> AKMAFTLADRVTEEMLADKAALVVEVVEENYHDAPIVGIAVVNEHGRFFLRPETALADPQFVAWLGDETKKKSMFDSKRAAVALKWKGIELCGVSFDLLLAAYLLDPAQGVDDVAAAAKMKQYEAVRPDEAVYGKGAKRAVPDEPVLAEHLVRKAAAIWELERPFLDELRRNEQDRLLVELEQPLSSILAEMEFAGVKVDTKRLEQMGKELAEQLGTVEQRIYELAGQEFNINSPKQLGVILFEKLQLPVLKKTKTGYSTSADVLEKLAPYHEIVENILHYRQLGKLQSTYIEGLLKVVRPDTKKVHTIFNQALTQTGRLSSTEPNLQNIPIRLEEGRKIRQAFVPSESDWLIFAADYSQIELRVLAHIA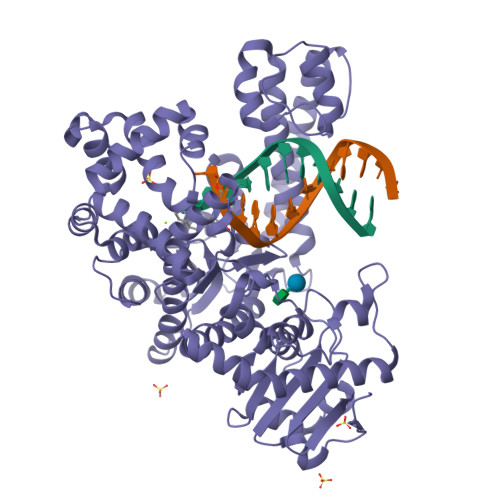EDDNLMEAFRRDLDIHTKTAMDIFQVSEDEVTPNMRRQAKAVNFGIVYGISDYGLAQNLNISRKEAAEFIERYFESFPGVKRYMENIVQEAKQKGYVTTLLHRRRYLPDITSRNFNVRSFAERMAMNTPIQGSAADIIKKAMIDLNARLKEERLQAHLLLQVHDELILEAPKEEMERLCRLVPEVMEQAVTLRVPLKVDYHYGSTWYDAK> MGSSHHHHHHSSGLVPRGSHMTTTISADQVNQIIYNLHHDPFEILGCHLLEEGKNTKKWVVRAYLPKAEAAWVIRPTERKEDPMNSVHHPNFFECIIETPELNHYQLKVKEGEHEKVIYDPYAFSSPYLTDEDIYLFSEGNHHRIYEKLGAHVGEINGVKGVYFAVWAPNARNVSVIGDFNNWDGREHQMRKRNYTIWELFVPEIGSGTVYKYEIKNSEGHIYEKSDPYGFYREVRPNTASIVVDIDNIYQWHDEEWLEKRRNSDPLKQPVSVYEVHLGSWLHGSSAEKMPLLNGEADPVIVSEWNPGARFLSYYELAEKLIPYVKDMGYTHI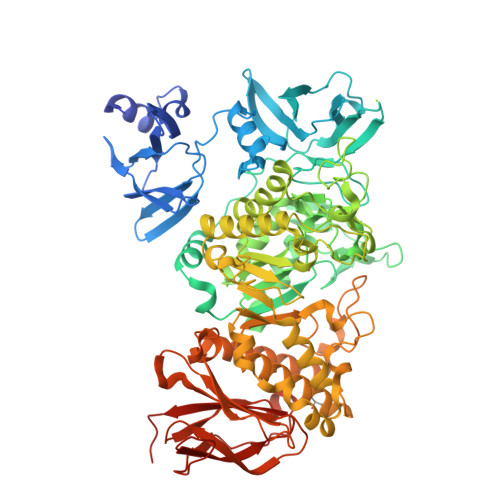ELLPIAEHPFDGSWGYQVTGFYSPTSRFGRPEDFMYFVDKCHENGIGVILDWVPGHFPKDSHGLAYFDGTHLYEHADPRIGEHKEWGTLVFNYGRHEVRNFLVANVLFWFDKYHVDGIRVDAVASMLYRNYLRKEGEWIANEYGGDEHIEAVSFIREVNTLLFEYFPGILSIAEESTEWEKVSRPVYDGGLGFNLKWDMGWMHDMLDYFNIDPYFRQYHQNNVTFSMAYYYNENFMLALSHDEIVHGKSNMLGKMPGDEWQKYANVRALFTYMYTHPGKKTMFMSMEFGQWSEWNVWGDLEWHLLQYEPHQQLKQFFTDLNALYQQEPALYTHDFEYHGFEAIDCNDNTHSVVSFLRRSDDPNDSLVVVCNFTPQPHSHYRIGVPEAGYYVELFNSDAKQYGGSNMGNLGGKWADEWSFHNKPYSLDLCLPPLAVLILKLDPTKVPEGTTIKEIAADEEE> MHNNENVSGISAYLLGLIIGDGGLYKLKYKGNRSEYRVVITQKSENLIKQHIAPLMQFLIDELNVKSKIQIVKGDTRYELRVSSKKLYYYFANMLERIRLFNMREQIAFIKGLYVAEGDKTLKRLRIWNKNKALLEIVSRWLNNLGV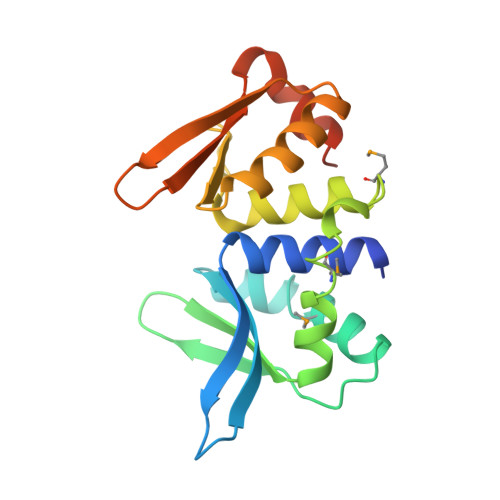RNTIHLDDHRHGVYVLNISLRDRIKFVHTILSSHLNPLPPE> M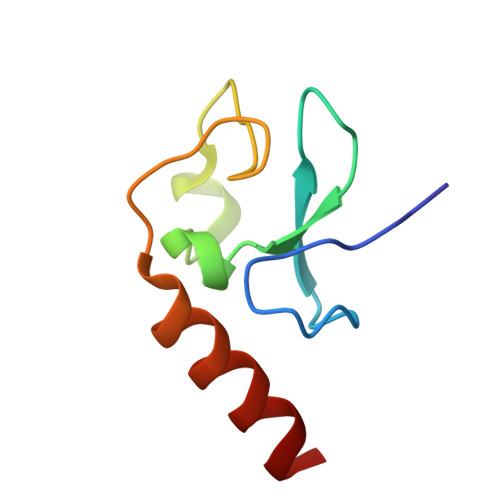GIITCICDLNDDDGFTIQCDHCNRWQHAICYGIKDIGMAPDDYLCNSCDPREVDINLARKIQQERINVK Methylenetetrahydrofolate dehydrogenase/cyclohydrolase 2 (MTHFD2) is a bifunctional metabolic enzyme found in mitochondria, exhibiting both dehydrogenase and cyclohydrolase catalytic activities. In one-carbon metabolism, MTHFD2 converts 5, 10-methylene tetrahydrofolate (5,10-CH2-THF) to 10-formyl tetrahydrofolate (10-CHO-THF) in mitochondria, thereby regulating the production of NADH, purines, and pyrimidines. An isozyme, methylenetetrahydrofolate dehydrogenase, cyclohydrolase and formyltetrahydrofolate synthetase 1 (MTHFD1), performs similar catalytic reactions to MTHFD2, albeit localized in the cytoplasm rather than the mitochondrion. The key distinction between these two proteins lie in their expression profiles: MTHFD1 is typically expressed in normal cells while MTHFD2 is abundantly expressed in immortal, embryonic, and cancer cells, but absent in adult normal cells.

In contrast, compound 16a and 16g, featuring 1H-tetrazole moiety substitution at the γ-carboxylic acid of glutamic acid, exhibited potent inhibition against MTHFD1. In comparison with the structure of MTHFD1/16e, the structure of MTHFD1/16g revealed that the 1H-tetrazole moiety shifted toward β strand h1 and was hydrogen bonded with Tyr240. Moreover, the larger size of the 1H-tetrazole moiety relative to the carboxylic acid group, in conjunction with its interaction with Tyr240, promoted a movement toward β strand h1 and therefore formed van der Waals interactions with Val252 and Leu51. These structural changes facilitated an interaction network that increased the binding affinity of 16g with MTHFD1. As a result, 16g demonstrated potent inhibitory effects on MTHFD1, hence exhibiting reduced selectivity toward MTHFD2. The superimposition of MTHFD1/16g and MTHFD2/16g revealed that the triaminopyrimidine headgroup, urea linker, and central phenyl ring of compound 16g aligned well in both structures. The important interactions between the headgroup and urea linker of 16g with residues Val131, Gln132, Leu133, Asp155, and Lys88 in MTHFD2 were retained in MTHFD1, where they corresponded to Val99, Gln100, Leu101, Asp125, and Lys56. The differences between these two structures were attributed to the residue substitutions from Ser83 and Asn87 in MTHFD2 to Leu51 and Val55 in MTHFD1. These hydrophobic residue replacements in MTHFD1 prevented the formation of hydrogen bonds with the amide or 1H-tetrazole moiety of 16g. Instead, a hydrogen bond was formed between the 1H-tetrazole moiety and Tyr240 in MTHFD1.

>[4x]APAEILNGKEISAQIRARLKNQVTQLKEQVPGFTPRLAILQVGNRDDSNLYINVKLKAAEEIGIKATHIKLPRTTTESEVMKYITSLNEDSTVHGFLVQLPLDSENSINTEEVINAIAPEKDVDGLTSINAGRLARGDLNDCFIPCTPKGCLELIKETGVPIAGRHAVVVGRSKIVGAPMHDLLLWNNATVTTCHSKTAHLDEEVNKGDILVVATGQPEMVKGEWIKPGAIVIDCGINYVPDDKKPNGRKVVGDVAYDEAKERASFITPVPGGVGPMTVAMLMQSTVESAKRFLEKFKPGLEHHHHHH>AGSMKLLNIKINEFAVTANTEAGDELYLQLPHTPDSQHSINHEPLDDDDFVKEVQEICDEYFGKGDRTLARLSYAGGQAYDSYTEEDGVYT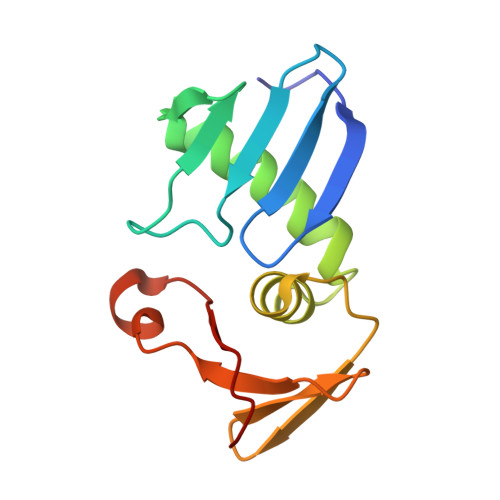TNTGDQFVEHSYADYYNVEVYCKADLV[8x]> NSVNPCCDPQTCKPIEGKHCISGPCCENCYFLRSGTICQRARGDGNNDYCTGIT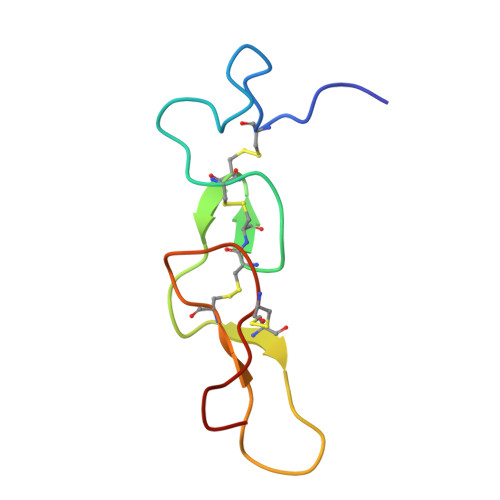PDCPRNRYNV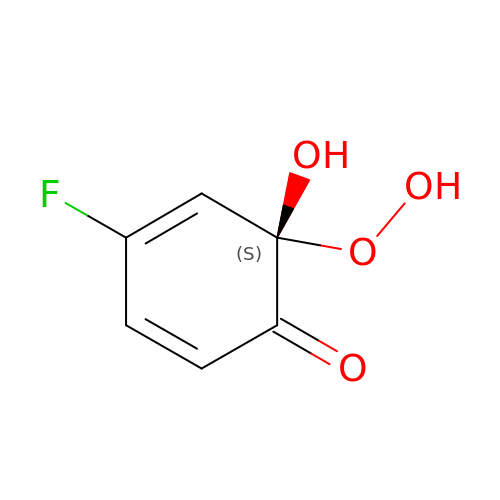(6S)-4-fluoro-6-hydroperoxy-6-hydroxycyclohexa-2,4-dien-1-one | C6 H5 F O4 | PXCVJIFNQFIHTP-LURJTMIESA-N Human paternally expressed gene 3 protein (PEG3) is a large multi-functional protein of nearly 1600 amino acids with a mass of about 165 kDa. Consistent with the presence of a large number of zinc fingers, PEG3 has been shown to bind DNA in a sequence specific manner, and has been detected predominantly in the nucleus, supporting the notion it is a bone fide transcription factor. PEG3 contains a SCAN domain near the N-terminus. The domain functions as a protein-protein interaction motif, mediating self-interaction and binding other proteins.

Here, we report the structure of the isolated SCAN homodimer from the human PEG3 protein (PEG3-SCAN). Crystals of human PEG3-SCAN belong to space group P65, with a VM value of 2.44 Å3 Da−1 and solvent content of approximately 50% for an asymmetric unit comprising two polypeptide chains. The crystals diffract to a resolution of 1.95 Å and the majority of the residues are located within well-defined electron density, apart from a few residues at the C-terminus. The human PEG3-SCAN domain folds as an extended V-shaped structure, with approximate overall dimensions of 50×25×25 Å. Helices α1 and α2 which form an N-terminal sub-domain are aligned antiparallel to create one half of the V. A C-terminal sub-domain, which forms the other half, results from α3, α4 and α5 being packed together. The domain aligns with the N-terminal sub-domains interacting with partner C-terminal sub-domains to form a dimer with approximate dimensions of 50×37×30 Å. The free energy of dissociation (ΔGdiss) is estimated as 19.4 kcal mol−1, and suggests that this assembly is thermodynamically stable, consistent with the observation of a stable dimer in solution. The human PEG3-SCAN homodimer is held together by an extensive network of hydrogen-bonding, salt-bridge interactions and van der Waals forces. The majority of these intermolecular contacts are formed between α1 and α2 (the N-terminal sub-domain) of one subunit and α3 on the C-terminal sub-domain of the partner. A hydrophobic patch comprising Phe49, Trp74, Leu75, Ile85, Ile86 and Leu89, from α2 and α3, make van der Waals interactions to equivalent residues in the partner subunit.

>[2x]GHMTDSEFFHQRFRNLIYVEFVGPRKTLIKLRNLCLDWLQPETRTKEEIIELLVLEQYLTIIPEKLKPWVRAKKPENCEKLVTLLENYKEMYQP>[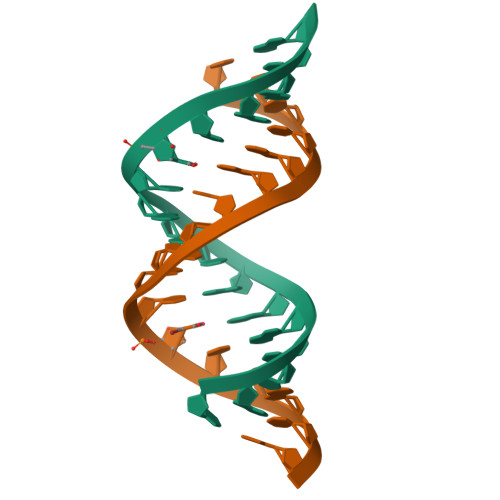2x]CACCGGAUGGUUCGGUG>MPVPNPTMPVKGAGTTLWVYKGSGDPYANPLSDVDWSRLAKVKDLTPGELTAESYDDSYLDDEDADWTATGQGQKSAGDTSFTLAWMPGEQGQQALLAWFNEGDTRAYKIRFPNGTVDVFRGWVSSIGKAVTAKEVITRTVKVTNVGRPSMAEDRSTVTAATGMTVTPASTSVVKGQSTT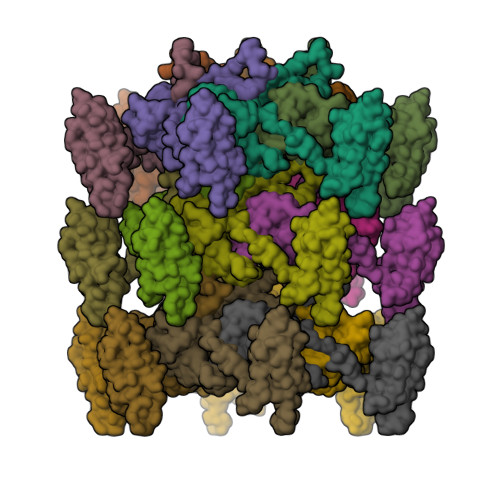LTVAFQPEGVTDKSFRAVSADKTKATVSVSGMTITVNGVAAGKVNIPVVSGNGEFAAVAEITVTAS[18x]>[2x]SPQHYTYLKEFRTEQCPLFVQHKCTQHRPY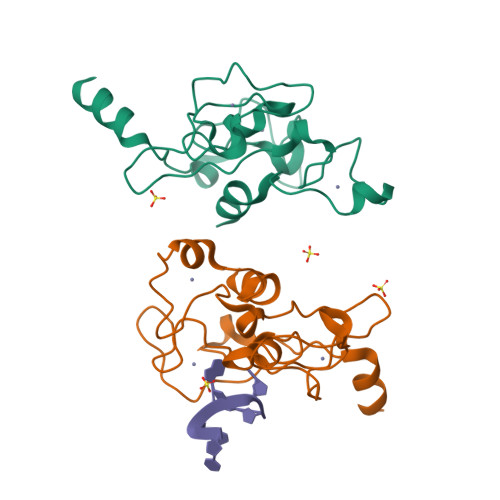TCFHWHFVNQRRRRSIRRRDGTFNYSPDVYCTKYDEATGLCPEGDECPFLHRTTGDTERRYHLRYYKTGICIHETDSKGNCTKNGLHCAFAHGPHDLRSPVYDIRELQAMEALQN> MG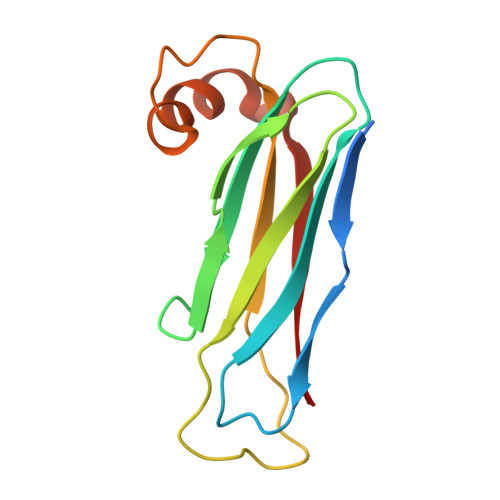SSHHHHHHMSAVEISPDVLVYKSPLTEQSTEYASISNNSDQTIAFKVKTTAPKFYCVRPNAAVVAPGETIQVQVIFLGLTEEPAADFKCRDKFLVITLPSPYDLNGKAVADVWSDLEAEFKQQAISKKIKVKYL N,N'-(1,4-phenylene)diacetamide 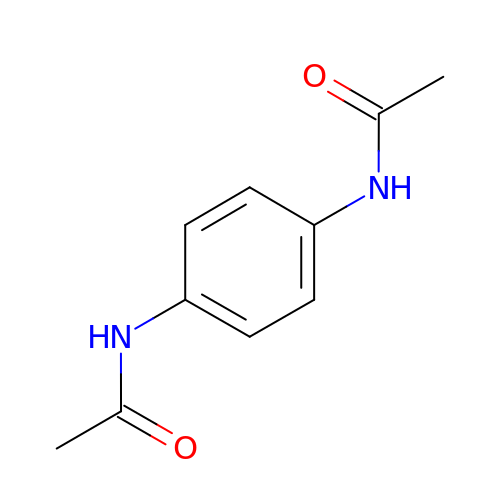| C10 H12 N2 O2 | KVEDKKLZCJBVNP-UHFFFAOYSA-N>MNLKDKILGVAKELFIKNGYNATTTGEIVKLSESSKGNLYYHFKTKENLFLEILNIEESKWQEQWKKEQIKAKTNREKFYLYNELSLTTEYYYPLQNAIIEFYTEYYKTNSINEKMNKLENKYIDAYHVIFKEGNLNGEWSINDVNAVSKIAANAVNGIVTFTHEQNINERIK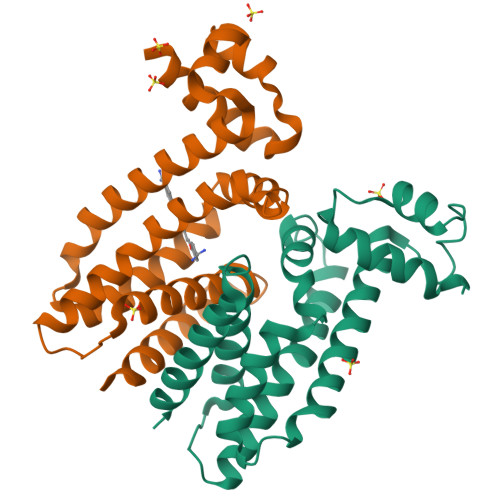LMNKFSQIFLNGLSK[4x]> MGKDYQVLGKNKVKVDSLEKVMGTAKFAADYSFPDMLYAGVFRSTVPHARIVSLDLSKARAIDGVEAVLDYHAIPGKNRFGIIIKDEPCLVDDKVRRYGDAIAVVAAQTPDLVQEALDAITIEY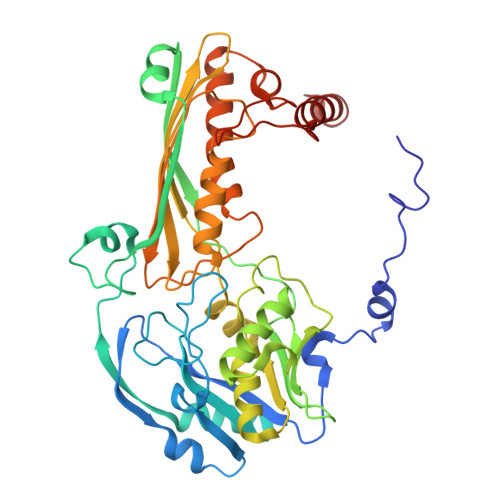EELEGIFTMERALEEDSPAIHGDTNIHQVKHLEYGDVDAAFKQCDIVVEDTYSTHRLTHMFIEPDAGVSYYDNEGMLTVVVSTQNPHYDRGEVAGMLALPNSKVRIIQATTGGGFGGKLDLSVQCHCALLTYHTKKPVKMVRSREESTTVSSKRHPMTMHCKTGATKDGRLQAVQVEMFGDTGAYASYGPAVITRATVHCMGPYVVPNVRVDAKFVYTNNPMSGAFRGFGVPQASVCHEGQMNALAKALGMDPIDIRILNAHQVGAKLATGQVLENSVGLIETLEKAREKAVEVMGYEKTR>GSGPSDMFVHTRDAIYKCAHLTNPTDETILLA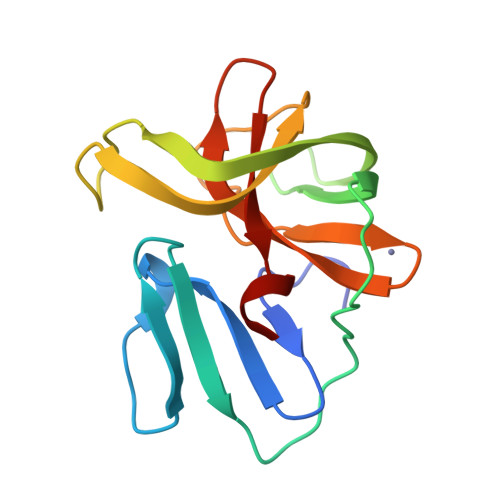LTADLQVDSTNVPGPDVIPCCDCTAGCYYSRSKDRYFPVECVSHDWYEIQESGYYPKHIQYNLLIGEGHCEPGDCGGKLLCKHGVIGMITAGGDNHVAFTDLRPYSS[4x]> MSRKKMGLLVMAYGTPYKEEDIERYYTHIRRGRKPEPEMLQDLKDRYEAIGGISPLAQITEQQAHNLEQHLNEIQDEITFKAYIGLKHIEPFIEDAVAEMHKDGITEAVSIVLAPHFSTFSVQSYNKRAKEEAEKLGGLTITSVESWYDEPKFVTYWVDRVKETYASMPEDERENAMLIVSAASLPEKIKEFGDPYPDQLHESAKLIAEGAGVSEYAVGWQSEGNTPDPWLGPDVQDLTRDLFEQKGYQAFVYVPVGFVADHLEVLYDN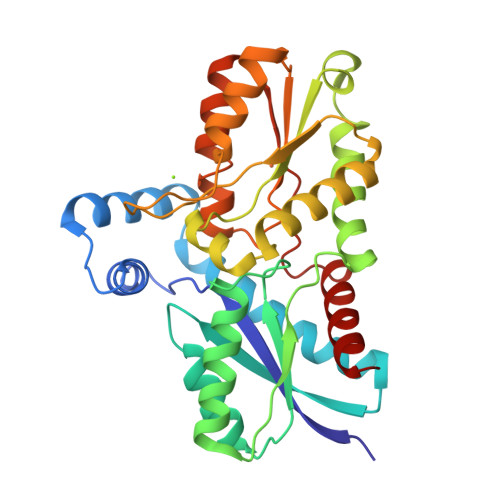DYECKVVTDDIGASYYRPEMPNAKPEFIDALATVVLKKLGR> INIGNKTNENVISFFDSTDAETQNHNALMKGCGEFIVNLRTLLRTFRTITDNWILQANTKTPITDLTNTTDAQGRDYMSYLSYLYRFYRGGRRYKFFNTTPLKQSQTCYIRSFLIPRNYSADEINVDGPSHITYPVINPVHEVEVPFYSQYRKIPIASTSDKGYDSSLMYFSNTATTQIVARAGNDDFTFGWMIGPPQLQGESRSVAP;> SENSVETQEITTFHDVETPNRIDTPMAQDTSSARNMDDTHSIIQFLQRPVLIDNIEIIAGTTADANKPLSRYVLDQQNSQKYVRSWTLPSTVLRAGGKAQKLANFKYLRCDVQVKLVLNANPFVAGRMYLAYSPYDDKVDTARSVLQTSRAGVTGYPGVELDFQLDNSVEMTIPYASFQEAYDLVTGTEDFVQLYLFPITPVLGPKSESESSKVDISVYMWLSNISLVIPTYRINP;> SKPRNQQQVCPLQNVPAWGYSLYKGIDMSVPLAYDPNNELGDLKDVFPSAVDEMAIGYVCGNPAVKHVLTWKTTDAIQKPIANGDDWGGVIPVGMPCYSKSIRTTRISATENRETEVMDAAPCEYVANMFSYWRATMCYRITVVKTAFHTGRLEIFFEPGVIPVKPTVNNIGPDQDRLTGAVAPSDNNYKYILDLTNDTEVTIRVPFVSNKMFLKTAGIYGANSENNWNFHESFSGFLCIRPVTKLMAPDTVSDNVSIVVWKWAEDVVVVEPKPLTSGPTQVYRPPPTASTAVEVLNVEL

Israeli acute bee paralysis virus (IAPV) is a member of the Aparavirus genus of the family Dicistroviridae. Viruses of the family Dicistroviridae have nonenveloped icosahedral capsids protecting linear, single-stranded, positive-sense RNA genomes of 8,500 to 10,200 nucleotides. The major capsid proteins VP1 to VP3 of IAPV form the capsid shell with pseudo-T=3 icosahedral symmetry, whereas VP4 is a small protein attached to the inner surface of the capsid. Here we present a high-resolution cryo-EM analysis of IAPV virions induced to release their genomes in vitro.

Genome release from IAPV virions results in the formation of empty capsids that are the same size as native virions. The structure of the empty capsid could be built except for residues 1 to 21 and 258 to 318 of VP2. There were no changes in the positions of subunits VP1 to VP3 relative to those in the native virus, and the structures of the icosahedral asymmetric units had a C-α atom RMSD of 0.98 Å. However, whole VP4 subunits and residues 1 to 21 of the N terminus of VP2 were not resolved for the empty capsids. As a consequence, the volume of the capsid cavity increased to 7.0 × 106 Å3. Furthermore, the loss of the structure of the VP2 N terminus resulted in a reduction in intrapentamer interfaces, from 5,900 Å2 to 5,150 Å2. However, the loss of the structure of the VP2 N terminus and of VP4 resulted in changes of the distribution of charges inside the capsids. Cryo-EM reconstruction of the empty IAPV capsid shows a strong electron density located on 5-fold axes close to the inner surface of the capsid, whereas the volume is occupied by VP4 subunits in the virions. We therefore speculate that the extra density belongs to positively charged ions, such as Ca2+ or Mg2+.>MPPNNSKYVLDPVSIKSVCGGEESYIRCVEYGKKKAHYSNLNLLAKAILAGMFVGLCAHASGIAGGLFYYHKLREIVGASMSVFVYGFTFPIAFMCIICTGSDLFTGNTLAVTMALYEKKVKLLDYLRVMTISLFGNYVGAVSFAFFVSYLSGAFTNVHAVEKNHFFQFLNDIAEKKVHHTFVECVSLAVGCNIFVCLAVYFVLTLKDGAGYVFSVFFAVYAFAIAGYEHIIANIYTLNIALMVNTKITVYQAYIKNLLPTLLGNYIAGAIVLGLPLYFIYKEHYYNFERSKRDNNDAQMKSLSIELRN[5x]

The P. falciparum lactate transporter PfFNT, encoded by pf3D7_0316600, belongs to the formate–nitrite transporter (FNT) family. After glucose is broken down into lactic acid by glycolysis inside the parasite, the end products, including lactate and protons, are extruded to the extraparasite milieu by PfFNT. The 5 protomers of PfFNT resemble as a pentagon-like homopentamer, with a width of approximately 80 Å and height of approximately 70 Å, with a 5-fold axis that is perpendicular to the membrane plane. Similar to the reported prokaryotic homologs, each protomer of PfFNT, comprising 6 transmembrane (TM) segments, presents a typical 3+3 invert repeat that is conserved throughout FNT family members.

Using C5 symmetry, we solved the structure of PfFNT to a final resolution of 2.3 Å. Owing to the high resolution, the polypeptide chain, including residues 7 to 293, of each protomer was unambiguously assigned to the density map. Although 250 mM sodium lactate was incubated with PfFNT before grid preparation, no extra density for lactate was found, which might be attributed to the low affinity between lactate and PfFNT. Similar to E. coli FocA (ecFocA), the pore radii of the extracellular constriction site for both apo and inhibitor-bound PfFNT are less than 1.5 Å, suggesting closure of the extracellular gate. The apo PfFNT tightly seals at this site with a pore radius of approximately 1 Å, whereas the inhibitor-bound structure opens to the cytoplasmic side. The central pore between 2 constriction sites is encompassed by hydrophobic residues except for 2 polar residues, Thr106 and His230, which are highly conserved in both prokaryotic and Plasmodium homologous. These 2 residues coordinate with each other through a hydrogen bond in the apo form PfFNT. Although the NTL is unstructured, 5 NTLs of each protomer orderly tangle to each other. The extra CTH protrudes into the cytoplasm of the parasite and is stabilized by 3 hydrogen bonds (Tyr8-His284, Glu30-Tyr285, and Lys120-Glu289). We captured an occluded apo form and an inward-open inhibitor-bound state.> SEFASMKRLSEIKVLPILESLKYIKHNHASVVRFGD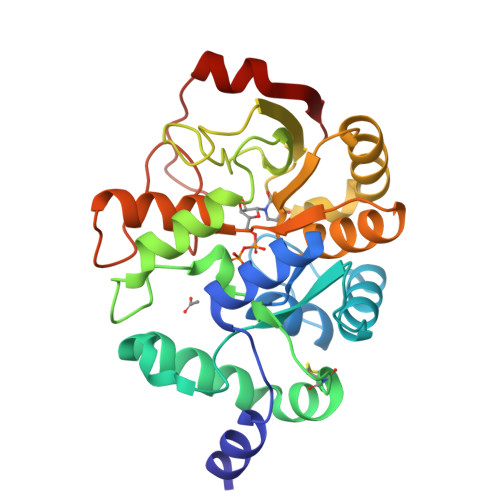GEIDLMTGHSIPYQDYNEKLAKRLQQILQTKSDEKLLVCLPDVFSNMDRYNQNARHFWERHFLKYSEFYLNCCDAPFYGSTFISRPYIDLIDKSPSEAYFESLKELWRGKDLLIVEGATSRSGVGNDLFVAASSIKRLVCPSKNAFQYYDEILRLTEKNAKNRLILVMLGPTAKVLVADLTTKGYQAIDLGHIDSEYEWYEMGATYKVKLTNKHTAEFNYDEGIELEFSQEYQEQIVARIG> MVFKIKDEWGEFLVRLARRAIEEYLKTGKEIEPPKDTPPELWEKMGVFVTLNRYNVPPQTALRGCIGFPTPIYPLVEATIKAAIYSAVDDPRFPPVKLEEMDNLVVEVSVLTPPEL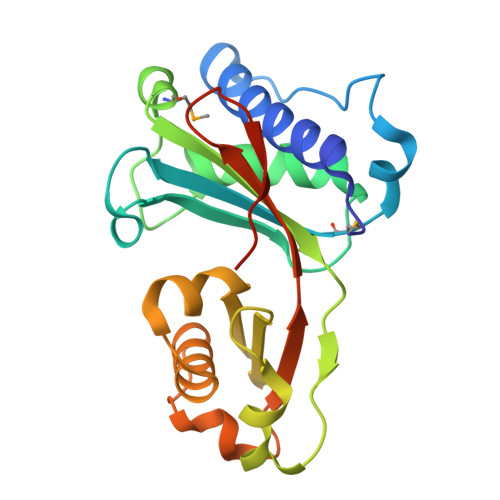IEGPPEERPRKIKVGRDGLIVEKGIYSGLLLPQVPVEWGWDEEEFLAETCWKAGLPPDCWLDEDTKVYKFTAEIFEEEYPRGPIKRKPLVLEHHHHHH The genome of malletwood is the only known plant genome that contains a gene coding for an α‐actinin‐like protein. The results clearly show that this protein has all properties of genuine α‐actinin. The R. argentea α‐actinin‐like protein dimerises in solution and thereby can cross‐link actin filaments. Based on these results, we believe the R. argentea protein represents a genuine α‐actinin, making R. argentea unique in the plant world.

In order to characterize its structure and function, we synthesized the gene and expressed the recombinant R. argentea protein. The N‐terminal actin‐binding domain (ABD), with two calponin homology motifs, is very similar to the ABD of any α‐actinin. The C‐terminal calmodulin‐like domain, as well as the intervening rod domain, are also similar to the corresponding regions in other α‐actinins.

> MTTVDGTANGNGAVPSTDYANGFNQNNGTSNVIDGNYMEQEEEWERAGLLDPAWEKQQRKTFTVWCNSHLRKADTQIENIEEDFRNGLKLMLLLEVISGETLPKPDRGKMRFHKIANVNKALDFIASKDVKLVSIGAEEIVDGNAKMTLGLIWTIILRFAIQDIEVEASTAKEGLLLWCQRKTSPYKNVNVHNFHNSWKDGLAFCALIHRHRPELIDYNSLTREDPVRNLNLAFDVAEKHLNIPKMLDAEDIKTSLKPDERAIMTYISSYYHTFANAQQA> MSMLKREDWYDLTRTTNWTPKYVTENELFPEEMSGARGISMEAWEKYDEPYKITYPEYVSIQREKDSGAYSIKAALERDGFVDRADPGWVSTMQLHFGAIALEEYAASTAEARMARFAKAPGNRNMATFGMMDENRHGQIQLYFPYANVKRSRKWDWAHKAIHTNEWAAIAARSFFDDMMMTRDSVAVSIMLTFAFETGFCNMQFLGLAADAAEAGDHTFASLISSIQTDESRHAQQGGPSLKILVENGKKDEAQQMVDVAIWRSWKLFSVLTGPIMDYYTPLESR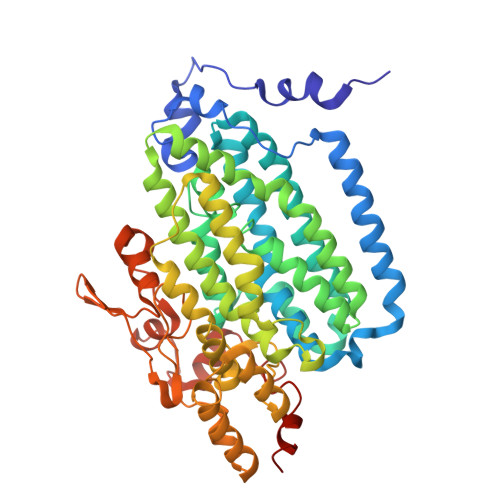NQSFKEFMLEWIVAQFERQLLDLGLDKPWYWDQFMQDLDETHHGMHLGVWYWRPTVWWDPAAGVSPEEREWLEEKYPGWNDTWGQCWDVITDNLVNGKPELTVPETLPTICNMCNLPIAHTPGNKWNVKDYQLEYEGRLYHFGSEADRWCFQIDPERYENHTNLVDRFLKGEIQPADLAGALMYMSLEPGVMGDDAHDYEWVKAYQKKTNAA> GSHMMIIVCASCDAKNRVPEEKLTAQPSCGQCHQPLLPLEPIELNEQNFSNYITNSDLPILIDLWAEWCGPCKMMAPHFAQVAKQNP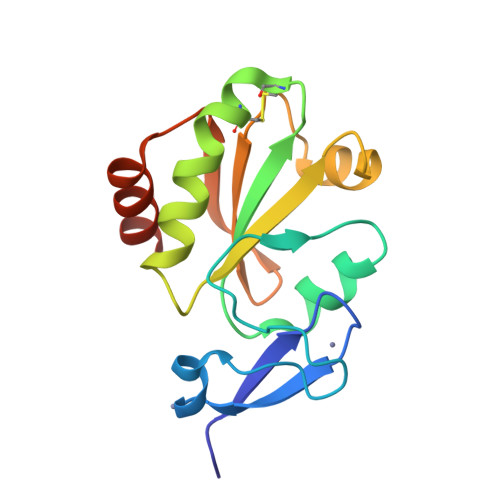RVIFAKINTEESPRLSQAFNVRSIPTLVLMNKTTEVARMSGALRAPELQQWLDQQLQTNFGS1-[3'-(trifluoromethyl)[1,1'-biphenyl]-2-yl]-1,3-dihydro-2H-pyrrol-2-one 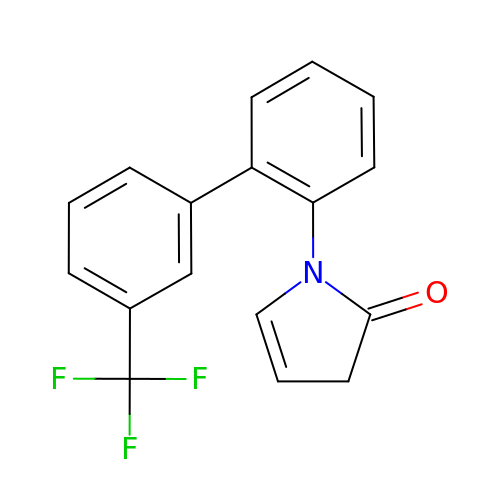| C17 H12 F3 N O | AIIYIYPODZMVSU-UHFFFAOYSA-N Langya virus (LayV) was recently found in shrews and isolated from febrile patients in China, representing the first human-infecting HNV from shrew origin. HNV infections are facilitated by the attachment glycoprotein (G) and the fusion glycoprotein (F). Upon G-mediated receptor engagement, F is triggered and promotes membrane fusion and viral entry. LayV F and G are closely related to MojV F and G but distantly related to their NiV and HeV counterparts.

CryoSPARC 3DFlex analysis reveals this 310-helix creates a hinge-like pivot point permitting a ~20° rotation of the membrane-proximal region relative to the head-interacting region of the stalk that could influence receptor-binding. Formation of the 310-helix results from K85 being oriented away from and L86 toward the core of the coiled coil, positioning them in hydrophilic and hydrophobic environments, respectively. To maintain α-helical integrity, K85 would need to orient toward and L86 away from the core of the coiled coil. The equivalent residues are conserved in MojV G, GAKV G, and DARV G whereas they are respectively hydrophobic and hydrophilic in distant HNVs. Therefore, the K85L/L86K mutations are expected to favor α-helical propensity in the LayV subgroup and LayV K85L/L86K GSM had a twofold enhanced production yield relative to LayV GSM. To further our understanding of the role of the K85L/L86K mutations on expression enhancement and rule out a possible impact of the oP4h tetramerization motif on the overall LayV G conformation, we determined a 3.2 Å resolution structure of the LayV K85L/L86K GSM without oP4h. The structure is virtually indistinguishable from LayV GSM with oP4h except for residues 82 to 89 which adopt a canonical α-helical structure instead of the 310-helix. These findings confirm that the designed K85L/L86K mutations restore the continuity of the α-helical stalk in this region, possibly explaining enhanced expression, and show that the positioning of the head domains relative to the stalk is most likely an intrinsic property of LayV G, which does not seem to be affected by stalk modifications.

>[4x]LKAIQAMLKIIQDEVNSLKEMLVSLDQLVKTEIKPKVSLINTAVSVSIPAQISNLQTKVLQKLVYLEESITKQCTXXXXXXXXXXXXXXXXXXXXXXXDTTDDDKVDTTIKPVEYYKPDGCNKTNDHFTMQPGVNFYTVPNLGPSSSSADECYTNPSFSIGSSIYMFSQEIRKTDCTTGEILSIQIVLGRIVDKGQQGPQASPLLVWSVPNPKIINSCAVAAGDETGWVLCSVTLTAASGEPIPHMFDGFWLYKFEPDTEVVAYRITGFAYLLDKVYDSVFIGKGGGIQRGNDLYFQMFGLSRNRQSIKALCEHGSCLXXXXGGYQVLCDRAVMSFGSEESLISNAYLKVNDVASGKPTIISQTFPPSDSYKGSNGRIYTIGERYGIYLAPSSWNRYLRFGLTPDISVRSTTWLKEKDPIMKVLTTCTNTDKDMCPEICNTRGYQDIFPLSEDSSFYTYIGITPSNEGTKSFVAVKDDAGHVASITILPNYYSITSATISCFMYKEEIWCIAVTEGRKQKENPQRIYAHSYRVQKMCFNI> MTTDNHQNDSVLDQQSGERTIDESNSISDENNVDNKREDVNVTSPTKSVSCISQAENGVA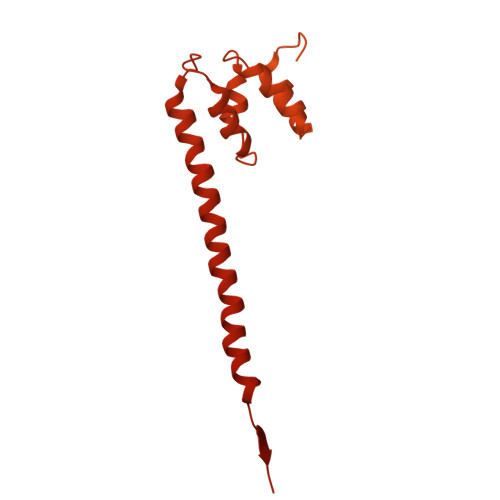SRTDESTITGSATDAETGDDDDDDDDDDDEDEDDEDEPPLLKYTRISQLPKNFFQRDSISSCLFGDTFFAFGTHSGILHLTTCAFEPIKTIKCHRSSILCINTDGKYFATGSIDGTVIIGSMDDPQNITQYDFKRPINSVALHSNFQASRMFVSGGMAGDVVLSQRNWLGNRIDIVLNKKKKKKTRKDDLSSDMKGPIMGIYTMGDLILWMDDDGITFCDVPTRSQLLNIPFPSRIFNVQDVRPDLFRPHVHFLESDRVVIGWGSNIWLFKVSFTKDSNSIKSGDSNSQSNNMSHFNPTTNIGSLLSSAASSFRGTPDKKVELECHFTVSMLITGLASFKDDQLLCLGFDIDIEEEATIDEDMKEGKNFSKRPENLLAKGNAPELKIVDLFNGDEIYNDEVIMKNYEKLSINDYHLGKHIDKTTPEYYLISSNDAIRVQELSLKDHFDWFMERKQYYKAWKIGKYVIGSEERFSIGLKFLNSLVTKKDWGTLVDHLNIIFEETLNSLDSNSYDVTQNVLKEWADIIEILITSGNIVEIAPLIPKKPALRKSVYDDVLHYFLANDMINKFHEYITKWDLKLFSVEDFEEELETRIEAASEPTASSKEEGSNITYRTELVHLYLKENKYTKAIPHLLKAKDLRALTIIKIQNLLPQYLDQIVDIILLPYKGEISHISKLSIFEIQTIFNKPIDLLFENRHTISVARIYEIFEHDCPKSFKKILFCYLIKFLDTDDSFMISPYENQLIELYSEYDRQSLLPFLQKHNNYNVESAIEVCSSKLGLYNELIYLWGKIGETKKALSLIIDELKNPQLAIDFVKNWGDSELWEFMINYSLDKPNFTKAILTCSDETSEIYLKVIRGMSDDLQIDNLQDIIKHIVQENSLSLEVRDNILVIINDETKKFANEFLKIRSQGKLFQVDESDIEINDDLNGVLDYKDDDDKDYKDDDDKDYKDDDDK5-HYDROXYMETHYL-3,4-DIHYDROXYPIPERIDINE 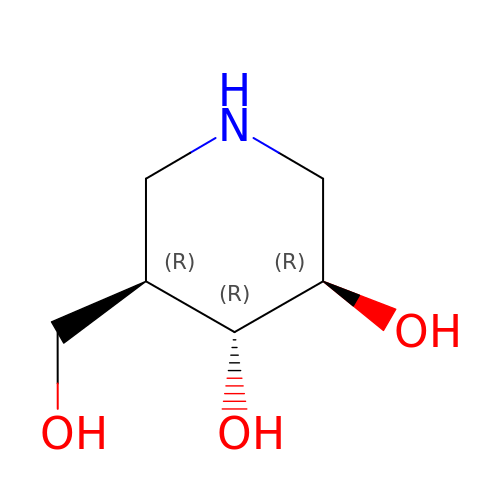| C6 H13 N O3 | QPYJXFZUIJOGNX-HSUXUTPPSA-N[[(2S,5R)-5-[4-azanyl-5-[2-(4-ethynylphenyl)ethynyl]-2-oxidanylidene-pyrimidin-1-yl]oxolan-2-yl]methoxy-oxidanyl-phosphoryl] phosphono hydrogen phosphate | C19 H20 N3 O12 P3 | 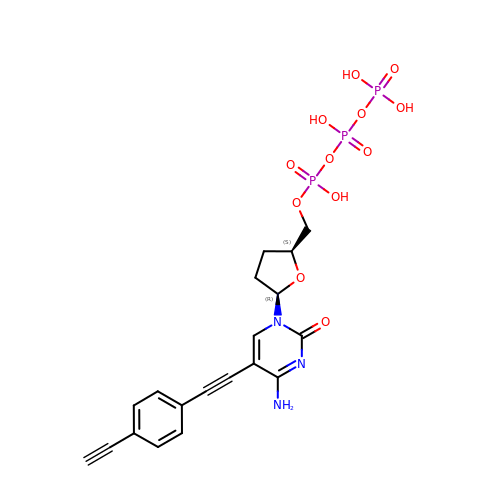PROFTMDIPXHDEG-DLBZAZTESA-N>[2x]AGMFRALFRQAVEDDRYGEFLDVLAEASAFRPQFASPEACSERLDPVLLAGGPTDRAEGRAVLVGCTGTAANGGPHEFLRLSTSFQEERDFLAVPLPGYGTGTGTGTALLPADLDTALDAQARAILRAAGDAPVVLLGHAGGALLAHELAFRLERAHGAPPAGIVLVDPYPPGHQEPIEVWSRQLGEGLFAGELEPMSDA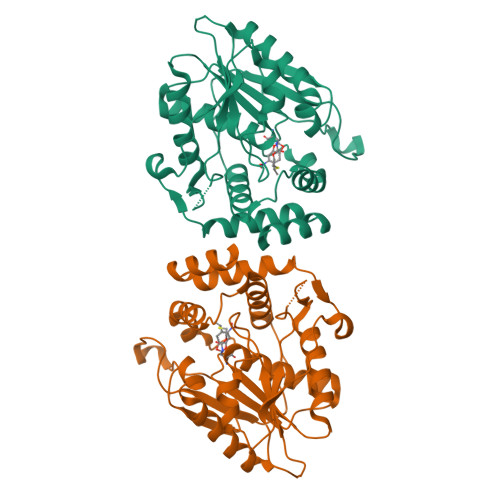RLLAMGRYARFLAGPRPGRSSAPVLLVRASEPLGDWQEERGDWRAHWDLPHTVADVPGDHFTMMRDHAPAVAEAVLSWLDAIEGIEGAGK>[2x]MAAAAVVAATVPAQSMGADGASSVHWFRKGLRLHDNPALLAAVRGARCVRCVYILDPWFAASSSVGINRWRFLLQSLEDLDTSLRKLNSRLFVVRGQPADVFPRLFKEWGVTRLTFEYDSEPFGKERDAAIMKMAKEAGVEVVTENSHTLYDLDRIIELNGQKPPLTYKRFQALISRMELPKKPAVAVSSQQMESCRAEIQENHDDTYGVPSLEELGFPTEGLGPAVWQGGETEALARLDKHLERKAWVANYERPRMNANSLLASPTGLSPYLRFGCLSCRLFYYRLWDLYKKVKR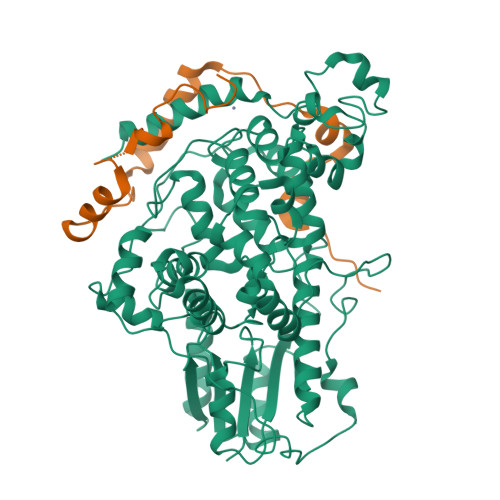NSTPPLSLFGQLLWREFFYTAATNNPRFDRMEGNPICIQIPWDRNPEALAKWAEGKTGFPWIDAIMTQLRQEGWIHHLARHAVACFLTRGDLWVSWESGVRVFDELLLDADFSVNAGSWMWLSCSAFFQQFFHCYCPVGFGRRTDPSGDYIRRYLPKLKGFPSRYIYEPWNAPESVQKAAKCIIGVDYPRPIVNHAETSRLNIERMKQIYQQLS;>SSDTSHTSKYFGSIDSSENNHKAKMIPDTEESEQFIKYVLQDPIWLLMANTDDSIMMTYQLPSRDLQAVLKEDQEKLKLLQRSQPRFTEGQRRELREVHPWVHTGGLPTAIDVTGCVYCES[2x]>MALTNAQILAVIDSWEETVGQFPVITHHVPLGGGLQGTLHCYEIPLAAPYGVGFAKNGPTRWQYKRTINQVVHRW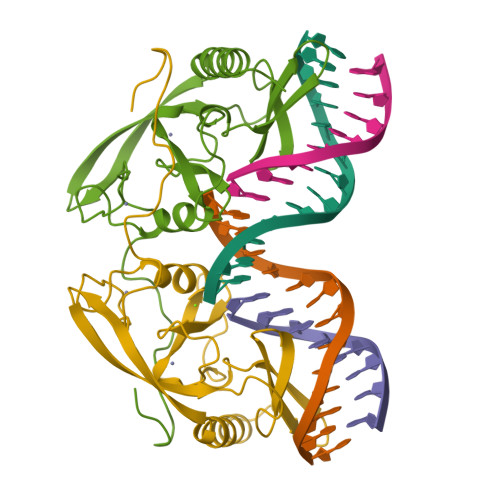GSHTVPFLLEPDNINGKTCTASHLCHNTRCHNPLHLCWESLDDNKGRNWCPGPNGGCVHAVVCLRQGPLYGPGATVAGPQQRGSHFVV[2x]>[2x]MGFEFTLMVVGESGLGKSTLINSLFLTDLYPERVIPGAAEKIERTVQIEASTVEIEERGVKLRLTVVDTPGYGDAINCRDCFKTIISYIDEQFERYLHDESGLNRRHIIDNRVHCCFYFISPFGHGLKPLDVAFMKAIHNKVNIVPVIAKADTLTLKE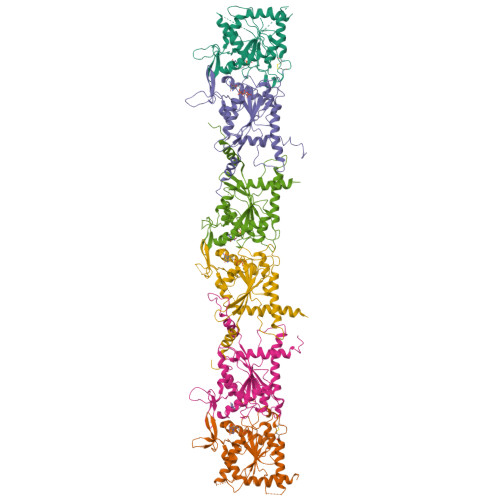RERLKKRILDEIEEHNIKIYHLPDAESDEDEDFKEQTRLLKASIPFSVVGSNQLIEAKGKKVRGRLYPWGVVEVENPEHNDFLKLRTMLITHMQDLQEVTQDLHYENFRSERLKRGG;>[2x]MAATDIARQVGEGCRTVPLAGHVGFDSLPDQLVNKSVSQGFCFNILCVGETGLGKSTLMDTLFNTKFEGEPATHTQPGVQLQSNTYDLQESNVRLKLTIVSTVGFGDQINKEDSYKPIVEFIDAQFEAYLQEELKIRRVLHTYHDSRIHVCLYFIAPTGHSLKSLDLVTMKKLDSKVNIIPIIAKADAISKSELTKFKIKITSELVSNGVQIYQFPTDDESVAEINGTMNAHLPFAVIGSTEELKIGNKMMRARQYPWGTVQVENEAHCDFVKLREMLIRVNMEDLREQTHTRHYELYRRCKLEEMGFKDTDPDSKPFSLQETYEAKRNEFLGELQKKEEEMRQMFVQRVKEKEAELKEAEKELHEKFDRLKKLHQDEKKKLEDKKKSLDDEVNAFKQRKTAAELLQSQGSQAGGSQTLKRDKEKKN;>MGSSHHHHHHSQDPMVAQQKNLEGYVGFANLPNQVYRKSVKRGFEFTLMVVGESGLGKSTLINSLFLTDLYSPEYPGPSHRIKKTVQVEQSKVLIKEGGVQLLLTIVDTPGFGDAVDNSNCWQPVIDYIDSKFEDYLNAESRVNRRQMPDNRVQCCLYFIAPSGHGLKPLDIEFMKRLHEKVNIIPLIAKADTLTPEECQQFKKQIMKEIQEHKIKIYEFPETDDEEENKLVKKIKDRLPLAVVGSNTIIEVNGKRVRGRQYPWGVAEVENGEHCDFTILRNMLIRTHMQDLKDVTNNVHYENYRSRKLAAVTYNGVDNNKNKGQLTKSPLAQMEEERREHVAKMKKMEMEMEQVFEMKVKEKVQKLKDSEAELQRRHEQMKKNLEAQHKELEEKRRQFEDEKANWEAQQRILEQQNSSRTLEKNKKKGKIF[2x]> MGSSHHHHHHSSGHMEQNPQSQLKLLVTRGKEQGYLTYAEVNDHLPEDIVDSDQIEDIIQMINDMGIQVMEEAPDADDLMLAENTADEDAAEAAAQVLSSVESEIGRTTDPVRMYMREMGTVELLTREGEIDIAKRIEDGINQVQCSVAEYPEAITYLLEQYDRVEAEEARLSDLITGFVDPNAEEDLAPTATHVGSELSQEDLDDDEDEDEEDGDDDSADDDNSIDPELAREKFAELRAQYVVTRDTIKAKGRSHATAQEEILKLSEVFKQFRLVPKQFDYLVNSMRVMMDRVRTQERLIMKLCVEQCKMPKKNFITLFTGNETSDTWFNAAIAMNKPWSEKLHDVSEEVHRALQKLQQIEEET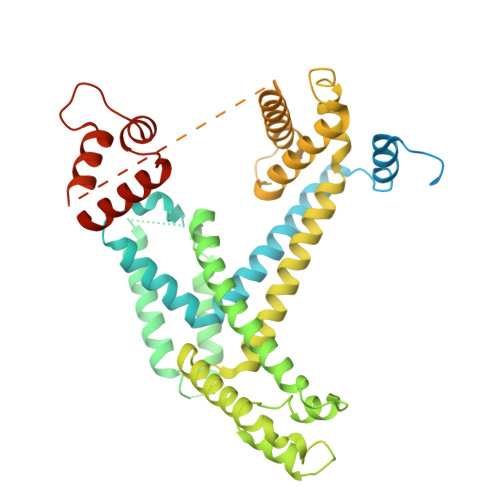GLTIEQVKDINRRMSIGEAKARRAKKEMVEANLRLVISIAKKYTNRGLQFLDLIQEGNIGLMKAVDKFEYRRGYKFSTYATWWIRQAITRSIADQARTIRIPVHMIETINKLNRISRQMLQEMGREPTPEELAERMLMPEDKIRKVLKIAKEPISMETPIGDDEDSHLGDFIEDTTLELPLDSATTESLRAATHDVLAGLTAREAKVLRMRFGIDMNTDYTLEEVGKQFDVTRERIRQIEAKALRKLRHPSRSEVLRSFLDD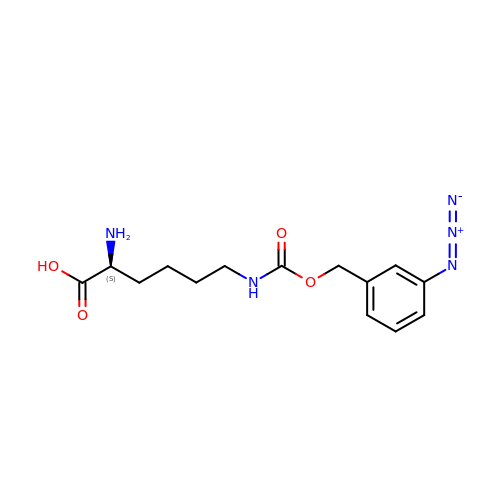N6-{[(3-azidophenyl)methoxy]carbonyl}-L-lysine | C14 H19 N5 O4 | HFCHIMDWTVTIEA-LBPRGKRZSA-N> MSSKYPRSVRRCLPLWALTLEAALILLFYFFTHYDASLEDQKGLVASYQVGQDLTVMAALGLGFLTSNFRRHSWSSVAFNLFMLALGVQWAILLDGFLSQFPPGKVVITLFSIRLATMSAMSVLISAGAVLGKVNLAQLVVMVLVEVTALGTLRMVISNIFNTDYHMNLRHFYVFAAYFGLTVAWCLPKPLPKGTEDNDQRATIPSLSAMLGALFLWMFWPSVNSPLLRSPIQRKNAMFNTYYALAVSVVTAISGSSLAHPQRKISMTYVHSAVLAGGVAVGTSCHLIPSPWLAMVLGLVAGLISIGGAKCLPVCCNRVLGIHHISVMHSIFSLLGLLGEITYIVLLVLHTVWNGNGMIGFQVLLSIGELSLAIVIALTSGLLTGLLLNLKIWKAPHVAKYFDDQVFWKFPHLAVGF;>MRFTFPLMAIVLEIAMIVLF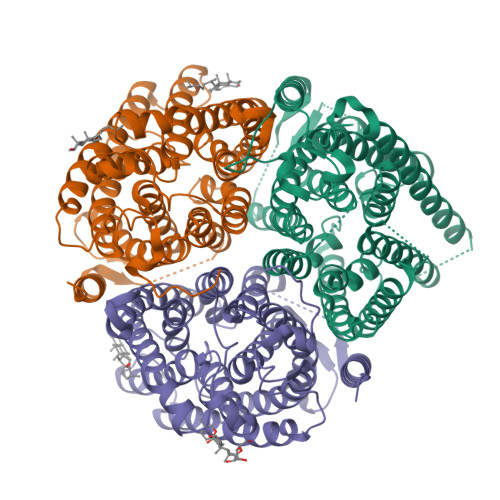GLFVEYETDQTVLEQLNITKPTDMGIFFELYPLFQDVHVMIFVGFGFLMTFLKKYGFSSVGINLLVAALGLQWGTIVQGILQSQGQKFNIGIKNMINADFSAATVLISFGAVLGKTSPTQMLIMTILEIVFFAHNEYLVSEIFKASDIGASMTIHAFGAYFGLAVAGILYRSGLRKGHENEESAYYSDLFAMIGTLFLWMFWPSFNSAIAEPGDKQCRAIVNTYFSLAACVLTAFAFSSLVEHRGKLNMVHIQNATLAGGVAVGTCADMAIHPFGSMIIGSIAGMVSVLGYKFLTPLFTTKLRIHDTCGVHNLHGLPGVVGGLAGIVAVAMGASNTSMAMQAAALGSSIGTAVVGGLMTGLILKLPLWGQPSDQNCYDDSVYWKVPKTR[2x]>AQYNYREVLQKSILFYAAQRSGQLPGNNPIDWRDDSALDDQGNGGEDLTGGWYDAGDHVKFGLPMAWTATTLIWGMIDLANGYGGDRNDAMQSVRWALDYFMKCHVSDNELYGQVGDGHADHAYWGRPEEMTMDRPAWSLTPSAPGSDLAGETAAALAAGSILFSDSDASYANQLLDHARTIYDFAYNNRGIYSESIPNAADFYRSSAYEDELCWGALWLYRATGEQDYMDKANEFLPQGRPWAFSWDSKE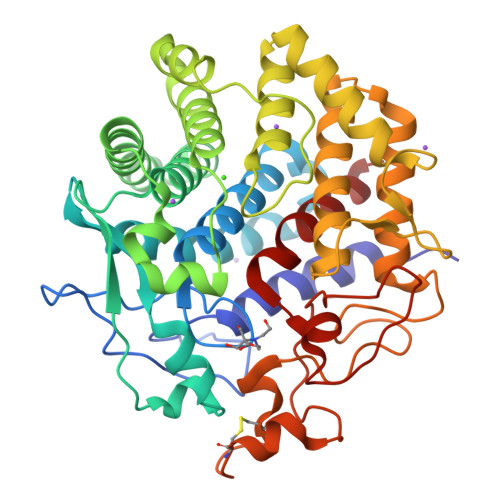AGSLVLLTSFGNSNARAQLEDFLQSWFPGGDIHYTPLGLAWRDTWGSLRYSANSAFIALLAAEEGVLTSQARTFARAQLDYMLGSTGRSFVVGFGTNPPLRPHHRAASCPDMPASCGWDQASDPAPNPQVLDGALVGGPDDQDNYNDDRQDYISNEVACDYNAGFQGALAGILQL[2x]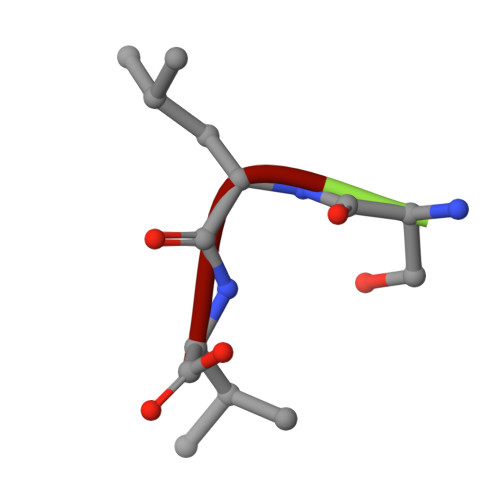> SLV>MTLEQAIERAGTKHGNKGWEAALSAIEMANLFKSLRGTGGSGSSMEIYEGKLTAEGLRFGIVASRFNHALVDRLVEGAIDSIVRHGGR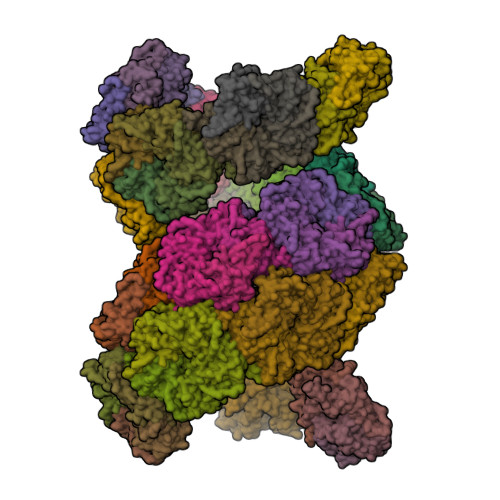EEDITLVRVPGSWEIPVAAGELARKEDIDAVIAIGVLIRGCTPHFDYIASEVSKGLANLSLELRKPITFGVITAD[100x]>[2x]MGSSHHHHHHSQGSMHYLDNLLLNTDSYKASHWLQYPPGTDASFFYVESRGGVYDQTAFFGLQSILKEAINRPVTHADIDDAKALLAAHGEPFNEAGWRDIVDRLGGQLPIRIRAVPEGCVVPTHNVLMTIESTDAKAFWVPSYLETLLLRVWYPVTVATVSWQVKQIVRDFLQRTSDDPEGQLPFKLHDFGARGVSSLGSAALGGAAHLV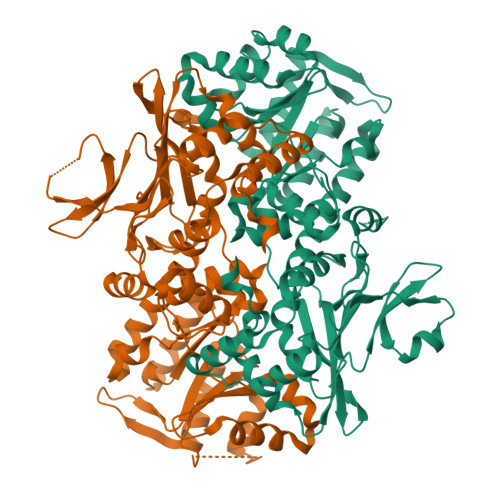NFLGTDTLSALLLARAHYHTPVAGYSIPAAEHSTITSWGREREVDAYRNMLTQFARPGAIVAVVSDSYDIYRAIREHWGTTLREEIIASGATVVIRPDSGDPVDVVEQCLLLLDEAFGHQVNGKGYKVLNHVRVIQGDGINPQSLRAILERITAAGYAADNVAFGMGGALLQKVDRDTQKFALKCSAVRVDGAWIDVYKDPITDQGKQSKRGRLTLLRDRATGQYRSALLDEVATHAGDSDDALVTVWENGQMLREWTLEQVRAHADAARL> GSMTEIALIGNPNSGKTSLFNLITGHNQRVGNWPGVSVERKSGLVKKNKDLEIQDLPGIYSMSPYSPEEKVARDYLLSQRADSILNVVDATNLERNLYLTTQLIETGIPVTIALNMIDVLDGQGKKINVDKLSYHLGVPVVATSALKQTGVDQVVKKAAHTTTSTVGDLAFPIYDDRLEAAISQILEVLGNSVPQRSA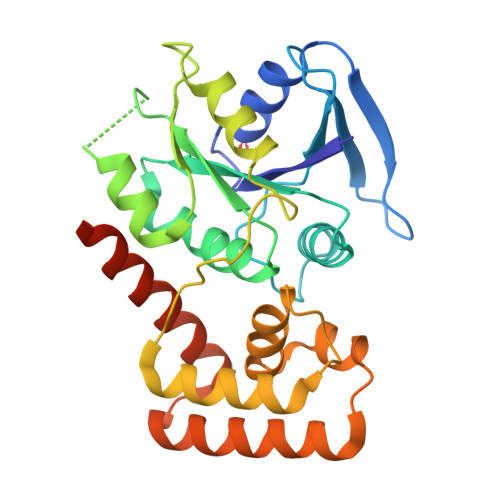RFYAIKLFEQDSLVEAELDLSQFQRKEIEDIIRITEEIFTEDAESIVINERYAFIERVCQMAESHTEDFALTLS>[83x]MELFDENYYAKAVANIIGEVKDPIMY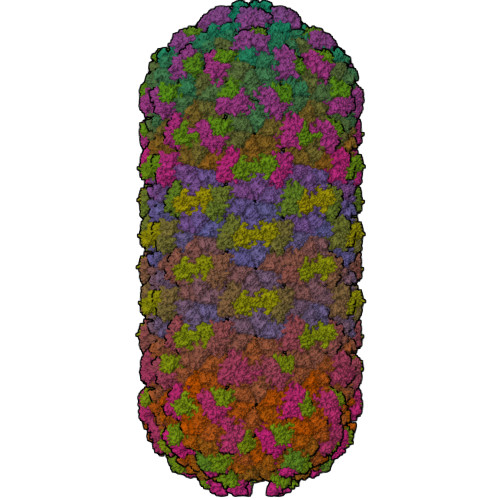KWFSPDQIEDVDLQMGYQKTVKWDAFLNANPTTIANEVNTISTIGFSSEVVRLNYLKLQYKFRHLKQTSEKFYTSDSYIGDINNNLLPFAQAYKLASSEIIKLINHFVLTGTVSIQKDGKNQKRLLPNMYGLLNMPEQIKEEVASGDKDKMDKIFEKIEAGLSKLELGDEFSTPMMVIVDPATSLKLVKPYAAAQGAASSCEKWEDVLIQTIKAINNREDVYIETSNLLKHKILIYPLNSELIKFKPSKYMLPTPNEQVDKDSTDVAHSYIDFVLGGLLATRKTILQVNIKQS;>MSDITKIKQEFDKKVAEIQALMKNPQQDSGLLSNSIDFRDQNLIFSNSGGVCTSSKDKIENYPAKGYPYKRGVKLSFGDGTTELEVEAGGGDDLYGVCSDIDEFSGMATVIPITNNFTGYLTLKKDGQNGVNPGDKLNFNQHGELEKVTGAQKSVNAIALSKAHKLTEDLFIVLASVFGNRAIKG[56x];> MALKGNMQVENLEAVEDPQVDLGAQVSAAPRAKRQARQAEDVQGEDPYLESISELDDVLLKFKKYSKSMSSIENKVFSSSSGCFKSKNERVDAYSFACSSYTDKIEEYLYDPANSFPYKRGVKLVPKENSIYVEVGADTDMYGICVDVCEFSCTAYVLPITNNFEGYLVTRNPSIKIGEILDINNNGVIIKAGGGPPTAINIYALSDSFTINFAPEDGNQDQNRYPRQEYSINLIKVAIFGNRGLEKTVNPDGG;>[26x]MGDTTQLVKEYQEKRSKLEKFMKNPQHDASLLSNSNEFRDKNVEFFASGGTRTSKFDKLENHPFLGYPYKRGVKRVIQEAQDNQSHYEPHVEAGGGEDLYGICIDIDEFSKTATIVPITNNFEGYLVAKDSTVKVKDKLIFNKDGALEKVTGAPNKATINATALTDAKQISNEVYLVKVAVFGNKAMSRN;>[83x]MTEKEEKEDLQAQDKEEQQIKADTKVISVQEFEEYMRFKEQANSKSKETSRDLSINERITKELAEVEERERIEKQLLLEAERINEIDTLAKAHLSNHFNKEVLLAKGYTLKDIMQAQRRELVRKFVPIEQIKAIAKVSDISHIDGEILEQLVSLAKVNIKLRKNASSSSSSVDSIKGNIAIKSEERASLLDSNFVPINFTEFVQAISNTYKQRRIQFYENLKRHKRTSIA3,6,9,12,15,18,21,24,27,30,33,36,39,42,45-pentadecaoxaoctatetracontane-1,48-diol | C33 H68 O17 | 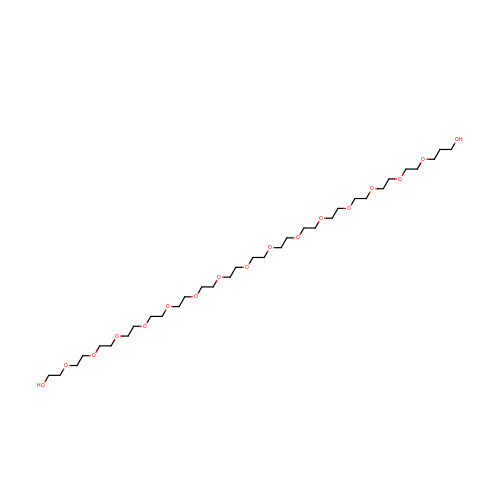UQGCHKWTTDVZHM-UHFFFAOYSA-N>MSLKIGIIGGGSVGLLCAYYLSLYHDVTVVTRRQEQAAAIQSEGIRLYKGGEEFRADCSADTSINSDFDLLVVTVKQHQLQSVFSSLERIGKT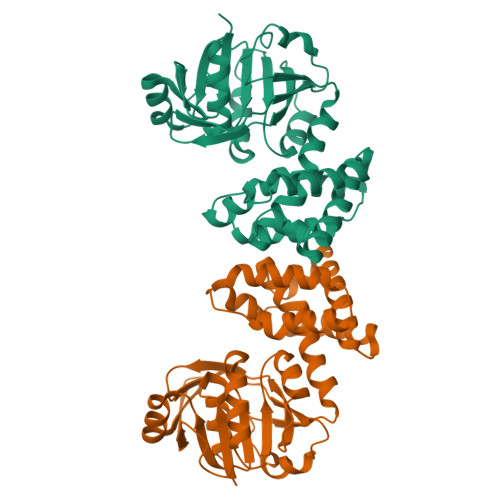NILFLQNGMGHIHDLKDWHVGHSIYVGIVEHGAVRKSDTAVDHTGLGAIKWSAFDDAEPDRLNILFQHNHSDFPIYYETDWYRLLTGKLIVNACINPLTALLQVKNGELLTTPAYLAFMKLVFQEACRILKLENEEKAWERVQAVCGQTKENRSSMLVDVIGGRQTEADAIIGYLLKEASLQGLDAVHLEFLYGSIKALERNTNKVEGHHHHHH[2x]> MIEADYLVIGAGIAGASTGYWLSAHGRVVVLEREAQPGYHSTGRSAAHYTVAYGTPQVRALTAASRAFFDNPPAGFCEHPLLSPRPEMVVDFSDDPEELRRQYESGKALVPQMRLLDAEQACSIVPVLRRDKVFGATYDPTGADIDTDALHQGYLRGIRRNQGQVLCNHEALEIRRVDGAWEVRCDAGSYRAAVLVNAAGAWCDAIAGLAGVRPLGLQPKRRSAFIFAPPPGIDCHDWPMLVSLDESFFLKPDAGMLLGSPANADPVEAHDVQPEQLDIATGMYLIEEATTL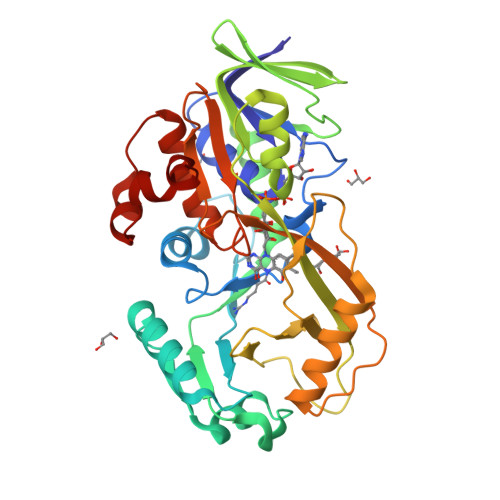TIRRPEHTWAGLRSFVADGDLVAGYAANAEGFFWVAAQGGYGIQTSAAMGEASAALIRHQPLPAHLREHGLDEAMLSPRRLSP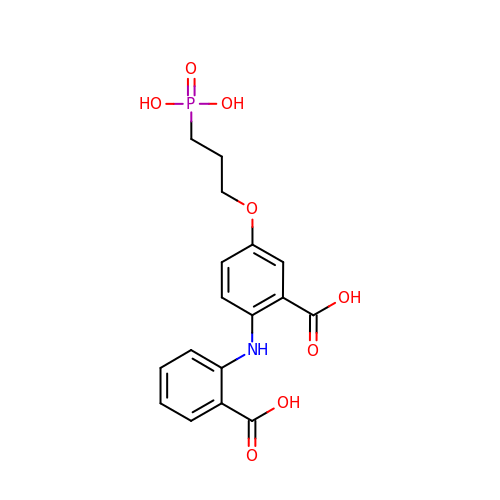2-[(2-carboxyphenyl)amino]-5-(3-phosphonopropoxy)benzoic acid | C17 H18 N O8 P | NQOSCSDORDCLER-UHFFFAOYSA-N>[2x]MRGSHHHH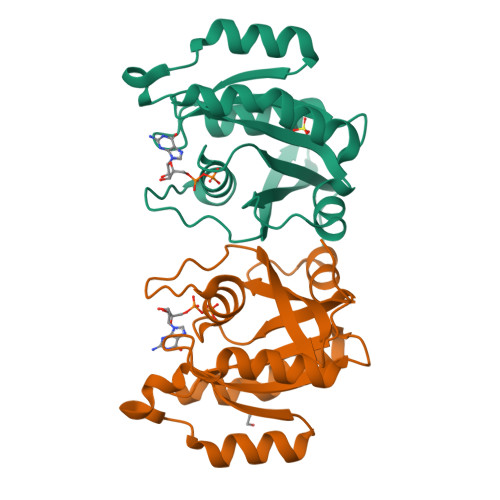HHGIPLPGRAMGTRDDEYDYLFKVVLIGDSGVGKSNLLSRFTRNEFNLESKSTIGVEFATRSIQVDGKTIKAQIWDTAGQERYRAITSAYYRGAVGALLVYDIAKHLTYENVERWLKELRDHADSNIVIMLVGNKSDLRHLRAVPTDEARAFAEKNGLSFIETSALDSTNVEAAFQTILTEIY> MGMSRSQSCFGYPLSIFFIVVNEFCERFSYYGMRALLILYFTLFIGWDDNLSTAIYHTFVALCYLTPILGALIADSWLGKFKTIVSLSIVYTIGQVVLAVSSINDLTDGNRDGTPDSLPVHVALSM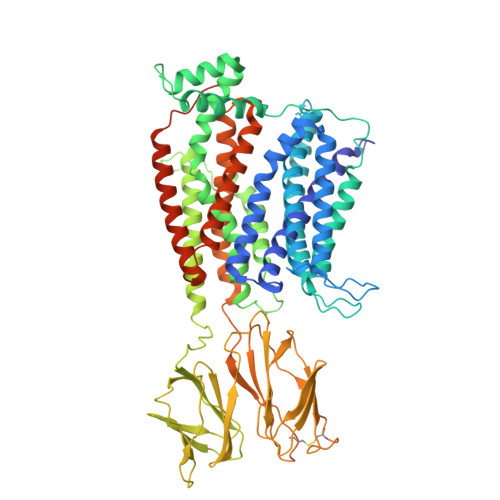IGLALIAFGTGGIKPCVSAFGGDQFEEGQEKQRNRFFSIFYLAINAGSLLSTIITPILRVQQCGIHSKQACYPLAFGVPAALMAVSLIVFVIGSRMYKKFQPQGNIMAKVAKCIGFAITNRIRHRSNKFPKREHWLDWAKEKYDERLISQIKMVTRVMFLYIPLPMFWALFDQQGSRWTLQATTMNGQIGVIEIQPDQMQTVNAILIVIMVPIMDAVVYPLIAKCGLNFTSLKKMTVGMFLASMAFVAAAIVQVEIDKTLPVFPNGHEVQVKVLNIGNNSMNISFPGETMAVNQMSQTGDFMTFDVDKLSINISSTGSPVTPVTHNFEQGHRHTILVWAPNHYRVIKDGLDRKPEKGQNGIRFVNAFDKSFDVTMDGTVYVNVTSHSASEYQFFPSGKKSFTINSTEISQQCERNFTSPRLGFGSAYTYVMGRKADGCPELSVFGDIPPNTVNMALQIPQYFLLTCGEVVFSVTGLEFSYSQAPSNMKSVLQAGWLLTVAVGNIIVLIVAGAGQFSKQWAEYILFAALLLVVCVIFGIMAQFYTYVNPAEVEAKFDDDEKKKNPEKENPYYTLDSVSQTRM>[4x]AWEIDPKDLTFLKELGTGQFGVVKYGKWRGQYDVAIKMIKE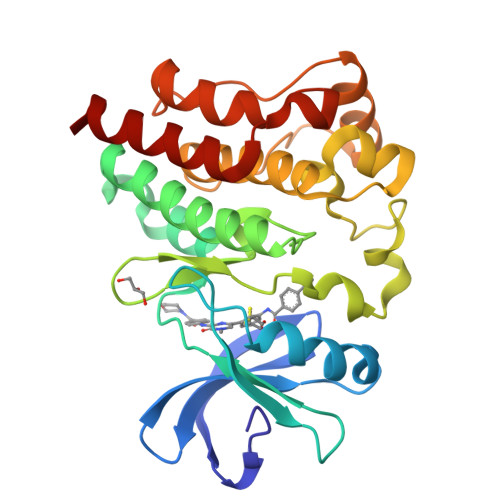GSMSEDEFIEEAKVMMNLSHEKLVQLYGVCTKQRPIFIITEYMANGCLLNYLREMRHRFQTQQLLEMCKDVCEAMEYLESKQFLHRDLAARNCLVNDQGVVKVSDFGMTRFVLDDEYTSSTGTKFPVKWASPEVLMYSKFSSKSDIWAFGVLMWEIYSLGKMPYERFTNSETAEHIAQGLRLPRPHLASERVYAIMYSCWHEKADERPTFKILLSNILDVMDEES> MLDAFSRVVVT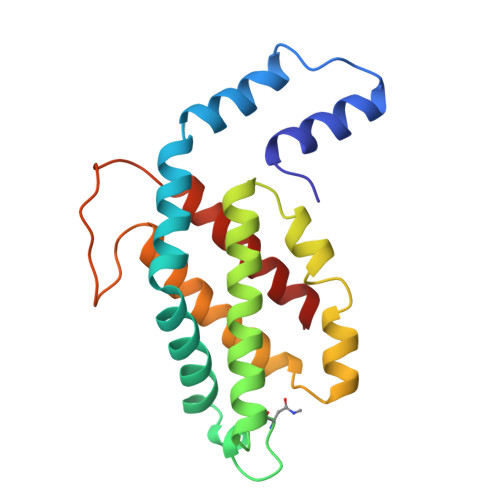SDAKAAYVGGSDLQSLKSFINDGNKRLDAVNYIVSNASCIVSDAVSGMICENPGLIAPGGNCYTNRRMAACLRDGEIILRYVSYALLAGDSSVLDDRCLNGLKETYIALGVPTASSSRAVSIMKATATAFITNTASGRKVEVAAGDCQALQAEAASYFDKVGSSID>MASPRAEQKQQTRHALMSAARHLMESGRGFGSLSLREVTRAAGIVPAGFYRHFSDMDQLGLALVAEVDETFRATLRAVRRNEFELGGLIDASVRIFLDAVGANRSQFLFLAREQYGGSLPIRQAIASLRQRITDDLAADLALLNKMPHLDGA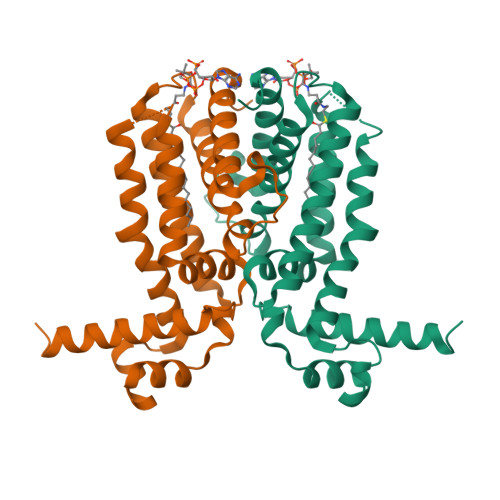ALDVFADLVVKTVFATLPELIDPPAADLPPHLMPAAKITHQLRFIMIGGKHWHGLPGSSVDKLAAALE[2x]> QNVQHQLAQFQQLQQQAQAISVQKQTVEMQINETQKALEELSRAADDAEVYK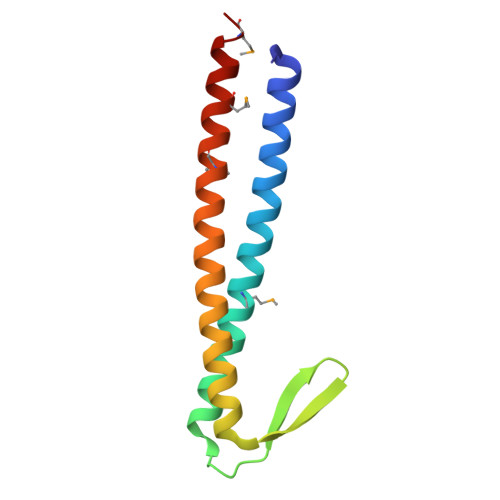SSGNILIRVAKDELTEELQEKLETLQLREKTIERQEERVMKKLQEMQVNIQEAMK>SNAMSVQNIVNINESNLQQTLEQSMTTPVLFYFWSERSQHCLQLTPVLESLAAQYHGQFILAKLDCDAEQMIAAQFGLRAIPTVYLFQNGQPVDGFQGPQPEEAIRALLDKVLPREEELKAQQAMQLMQEGNYIDALPLLKDAWQLSSQNSEIGLLLAEAQIALNRSEEAEAVLKTIPLQDQDTRYQGLVAQIELLKQAADTPEIQQLQQQVADNPQDAALATQLALQLHQVGRNEEALELLFSHLRKDLTAAEGQTRKT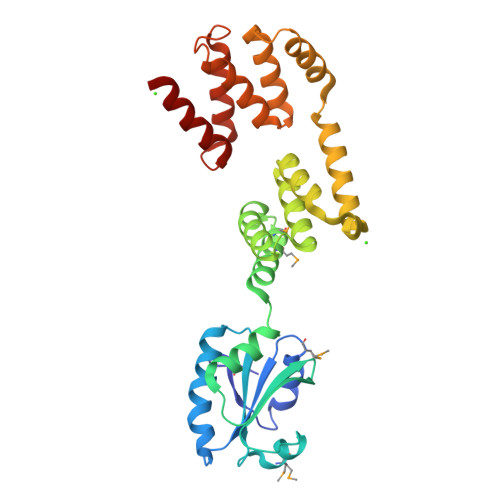FQEILAALGTGDALASKYRRQLYALLY[2x]>[2x]GNWDVNVNIEQNFIPDI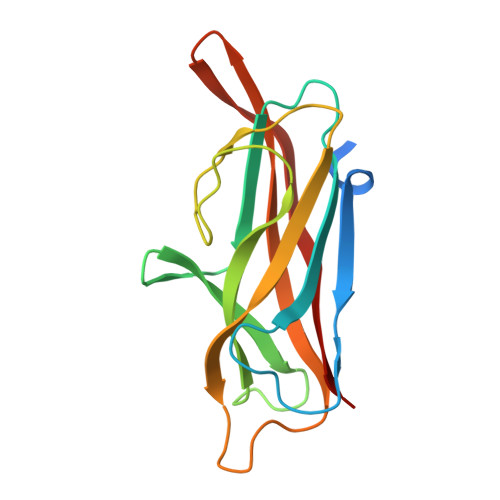DSAVRIIPVNYDSDPKLNSQLYTVEMTIPAGVSAVKIVPTDSLTSSGQQIGKLVNVNNPDQNMNYYIRKDSGAGKFMAGQKGSFSVKENTSYTFSAIYTGGEYPNSGYSSGTYAGHLTVSFYSNDNKQRTEIATKNFPVSTTIS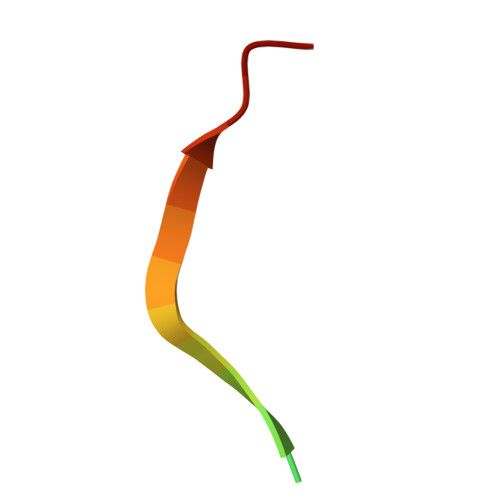> TEKEKGRLHCVEWTILER>[2x]RADPDPMKNTCKLLVVADHRFYRYMGRGEESTTTNYLIELIDRVDDIYRNTAWDNAGFKGYGIQIEQIRILKSPQEVKPGEKHYNMAKSYPNEEKDAWDVKMLLEQFSFDIAEEASKVCLAHLFTYQDFDMGTLGLAYGGSPRANSHGGVCPKAYYSPVGKKNIYLNSGLTSTKNYGKTILTKEADLVTTHELGHNFGAEHDPDGLAECAPNEDQGGKYVMYPIA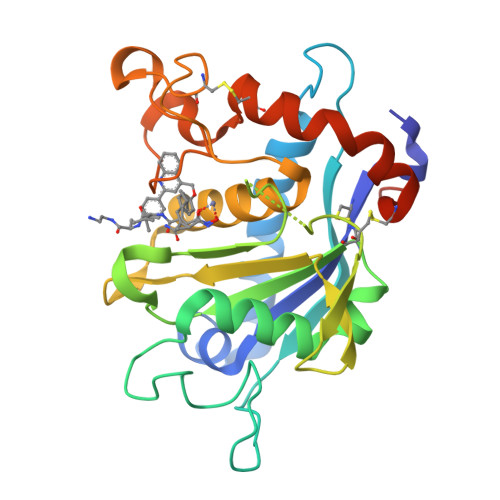VSGDHENNKMFSQCSKQSIYKTIESKAQECFQERSNKVGSHHHHHH>[15x]QVIEMNNSPLRDFVTWYSKQTGESVIVSPDVKGTVTVYSSDVKPENLRNFFISVLRANNFDMVGSNPSIIQKYNPNNQDYIDELPSSDNQEYDDNSAPSGGFFVPQNDNVTQTFKINNVRAKDLIRVVELFVKSNTSKSSNVLSVDGSNLLVVSAPKDILDNLPQFLSTVDLPTDQ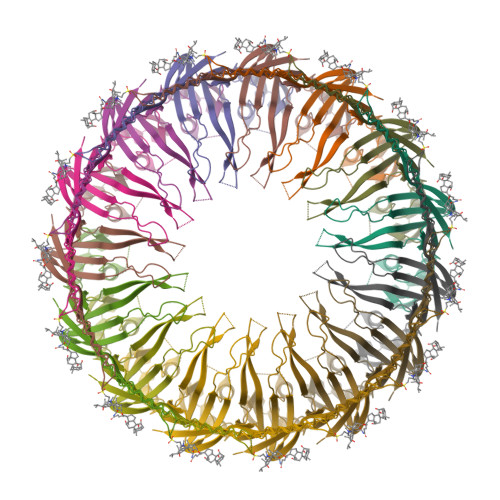ILIEGLIFEVQQGDALDFSFAAGSQRGTVAGGVNTDRLTSVLSSAGGSFGIFNGDVLGLSVRALKTNSHSKILSVPRILTLSGQKGSISVGQNVPFITGRVTGESANVNNPFQTVERQNVGISMSVFPVAMASAHHHHHHHGGNIVLDITIKADSLSSSTQASDVITNQRSIATTVNLRDGQTLLLGGLTDYKNTSQDSGVPFLSKIPLIGLLFSSRSDSNEESTLYVLVKATIVRAL>MHAALSTEVVHLRQRTEELLRCNEQQAAELETCKEQLFQSNMERKELHNTVMDLRGNIRVFCRIRPPLESEENRMCCTWTYHDESTVELQSIDAQAKSKMGQQIFSFDQVFHPLSSQSDIFEMVSPLIQSALDGYNICIFAYGQSGSGKTYTMDGVPESVGVIPRTVDLLFDSIRGYRNLGWEYEIKATFLEIYNEVLYDLLSNEQKDMEIRMAKNNKNDIYVSNITEETVLDPNHLRHLMHTAKMNRATASTAGNERSSRSHAVTKLELIGRHAEKQEISVGSINLVDLAGSESPKTSTRMTET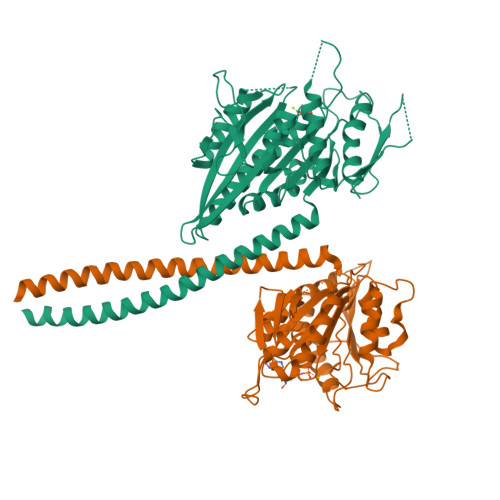KNINRSLSELTNVILALLQKQDHIPYRNSKLTHLLMPSLGGNSKTLMFINVSPFQDCFQESVKSLRFAASVNSCKMTK[2x]> SIITKSIVNADAEARYLSPGELDRIKSFVLSGQRRLRIAQILTDNRELIVKQGGQQLFQKRPDVVSPGGNAYGEEMTATCLRDLDYYLRLVTYGIVAGDVTPIEEIGLVGVKEMYNSLGTPISGVAEGVRSMKNVACSLLAGEDSAEAGFYFDYTLGAMQ;> MQDAITSVINAADVQGRYLDDNSLDKLRGYFQTGELRVRASATIAANAATIIKDSVAKALLYSDITRPGGNMYTTRRYAACIRDLDYYLRYATYGMLAGDPSILDERVLNGLKETYNSLGVPIGATIQAVQAMKEVTSSLVGPDAGKEMGVYFDYICSGLS

Components of phycobilisomes in Gracilaria chilensis are Phycobiliproteins (PBPs): Phycoerythrin (PE), and Phycocyanin (PC) in the rods, Allophycocyanin (APC) is found in the core, and linker proteins (L) present along the whole system. PBPs are chromophorylated proteins that share a general architecture. They are organized as heterodimers (αβ), which assembly themselves into trimers or hexamers. The subunits of PBPs are mono or multi chromophorylated with linear tetrapyrrols covalently bound to cysteine residues.

The pure protein was characterized by its spectroscopic properties of absorption (λAmax = 651nm) and emission (λEmax = 660nm) and the relationship A651/A280 as purity index. The purified APC was shown to contain only α and β subunits by mass spectrometry experiments. The result showed that Allophycocyanin from Gracilaria chilensis was purified in an oligomeric state (αβ)3. The final crystallization conditions were 2mg/mL protein concentration, 300mM NaCl, 20% v/v PEG 6000, and 100mM MES pH7. Crystals were diffracted at Soleil Synchrotron up to 2.3 Å resolution. The trimer for APC was obtained by crystallographic symmetry (P321). The biological unit is a trimer of heterodimers as it was determined by size exclusion chromatography. Indeed, α and β subunits contained one phycocyanobilin bound to cysteine 81 and are stabilized by Asn71, Arg83 and Asp84 in α subunit, and by methyl-Asn71 (Asm71) and Asp84 in β subunit.> SSQIRQNYSTEVEAAVNRLVNLYLRASYTYLSLGFYFDRDDVALCGV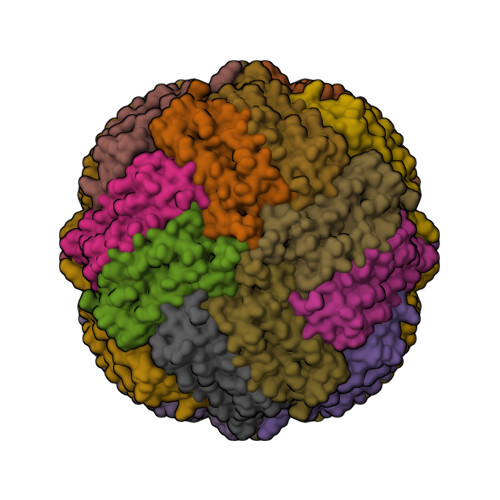AHFFRELAEEKREGAERLLKMQNQRGGRALFQDLQKPSQDEWGTTLDAMKAAIVLEKSLNQALLDLHALGSAQADPHLCDFLESHFLDEEVKLIKKMGDHLTNIQRLVGSQAGLGEYLFERLTLKHD> SMASQGGDSGNSKQESNSKDKEVKKIGITQLVEHPALDATRTGFVKALEKNGFKDGENIDIDFQNAQNDMPTTQSIASKFASDKKDLIFAISTPSAQAAFNATKDIPILITAVSDPVAAGLVKTLEKPGTNVSGTSDFVSVDKGLELLKIFAPKAKTIGVMYNTSEVNSKVQVDALKEYASKNGFKVVEKGITTSNEVNQGISSLVGKIDVLYVPTDNLVASSMPIVSKIATENKIPVIAAESGP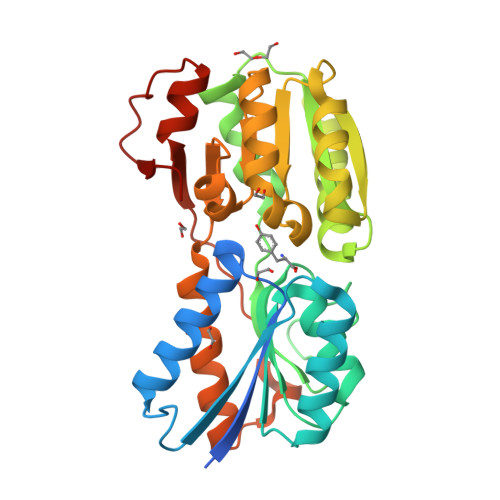VEKGALACQGINYEKLGYKTGEMAVKILNGESVSDMPVATSDDTDIIVNEDILKALGMEKPSNENISYVKTKQE> MAHHHHHHMFEHIDAYPGDPILTLNENFQKDPRDQKVNLSIGIYFDAEGRIPVMGAVREAETALQRDSGPKP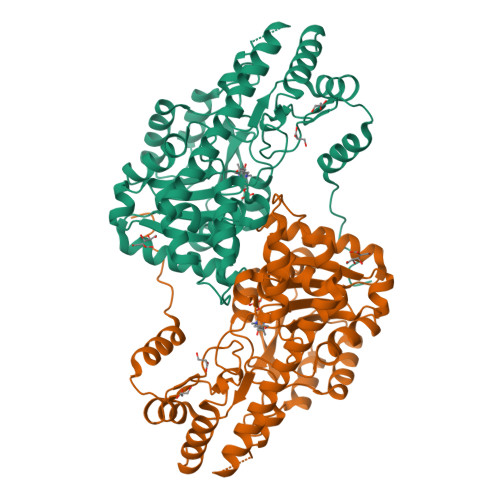YLPMVGLAAYRDAVQSLVFGADHPARAAGRIATLQTLGGSGALKVGADFLKRYFPDSQVWLSDPSWENHRFIFERAGFTVNTYPYYDEATGGLKFDAMLAAIDALPARSIVLLHACCHNPTGVDLDEGQWEKLIDVIEARELLPFVDMAYQGFGAGLDADAFAVRELARRGVPTLVANSFSKNFSLYGERVGGLSVVCEDAAAAERVLGQLAGAVRSNYSNPQTYGAKVVAAVLGTPALRKQWEEELSAMCRRIARMRQSIHDGLRDHVSGEALTRYVKQRGMFTYTGLTESQVDALREVHGVYILRSGRMCVAGLNDSNVGIVADAIGKVLKSGA>MKALRGMISEKGGWNLTVNNDNNTVVSSGGALDLSSGSKNLKIVKDGKKNNVTFDVAR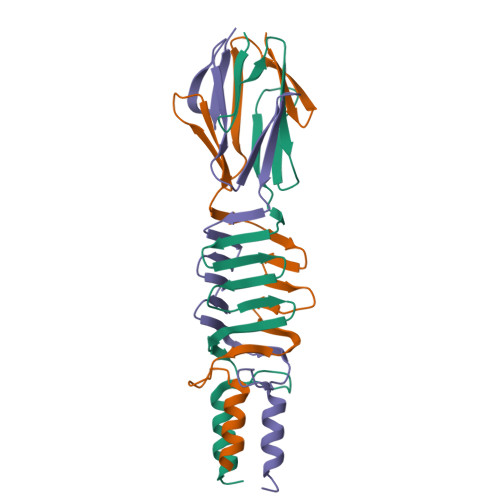DLTLKSIKLDGVTLNETGLFIANGPQITASGINAGSQKITGVAEGTDANDAVNFGQLKKIETEVKEQVAASGFVKQDSDTKYLTIGKDTDGDTINIANNKSDKRT[3x]>SVDLIGINVAGAEFTGGKLPGKHGTHYFFPPEGYFEYWSEQGIHTVRFPLKWERLQPSLNAELDDVYASL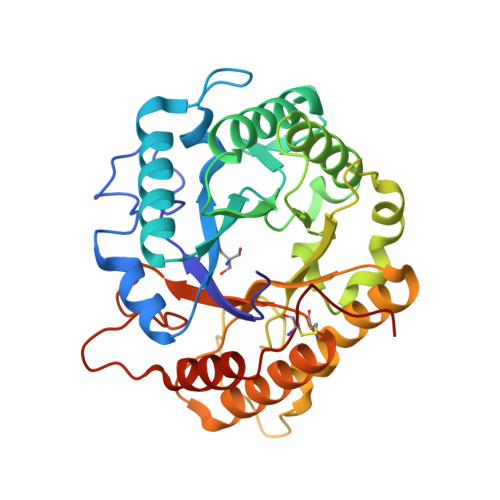VDDMLDQAKENDIKVILDVHNYARYRKKVIGTEDVPVSAYQDLMERIAKRWQGHDALFAYDIMNQPYGSADKLWPAAAQAGIDGVRKYDKKRPLLIEGASWSSAARWPRYADELLKLKDPADNMVFSAHVYIDEDASGSYKKGPGKDFEPMIGVKRVEPFVNWLKEHGKKGHIGEFGIPNDDERWLDAMDKLLAYLNENCIPINYWAAGPSWGNYKLSIEPKDGEKRPQVALLKKYAAKDNCSDFGPAKAE[2x]>[7x]DIVDYKDDDDKENLYFQGEPSQLPHCPSVSPSAQPWTHPGQSQLFADLSREELTAVM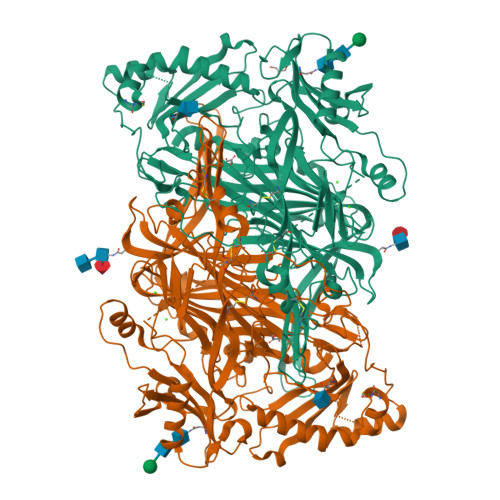RFLTQRLGPGLVDAAQARPSDNCVFSVELQLPPKAAALAHLDRGSPPPAREALAIVFFGRQPQPNVSELVVGPLPHPSYMRDVTVERHGGPLPYHRRPVLFQEYLDIDQMIFNRELPQASGLLHHCCFYKHRGRNLVTMTTAPRGLQSGDRATWFGLYYNISGAGFFLHHVGLELLVNHKALDPARWTIQKVFYQGRYYDSLAQLEAQFEAGLVNVVLIPDNGTGGSWSLKSPVPPGPAPPLQFYPQGPRFSVQGSRVASSLWTFSFGLGAFSGPRIFDVRFQGERLVYEISLQEALAIYGGNSPAAMTTRYVDGGFGMGKYTTPLTRGVDCPYLATYVDWHFLLESQAPKTIRDAFCVFEQNQGLPLRRHHSDLYSHYFGGLAETVLVVRSMSTLLNYDYVWDTVFHPSGAIEIRFYATGYISSAFLFGATGKYGNQVSEHTLGTVHTHSAHFKVDLDVAGLENWVWAEDMVFVPMAVPWSPEHQLQRLQVTRKLLEMEEQAAFLVGSATPRYLYLASNHSNKWGHPRGYRIQMLSFAGEPLPQNSSMARGFSWERYQLAVTQRKEEEPSSSSVFNQNDPWAPTVDFSDFINNETIAGKDLVAWVTAGFLHIPHAEDIPNTVTVGNGVGFFLRPYNFFDEDPSFYSADSIYFRGDQDAGACEVNPLACLPQAAACAPDLPAFSHGGFSHN2,2'-[(4-fluorobenzene-1,2-diyl)bis(oxy)]bis(5-nitrobenzonitrile) 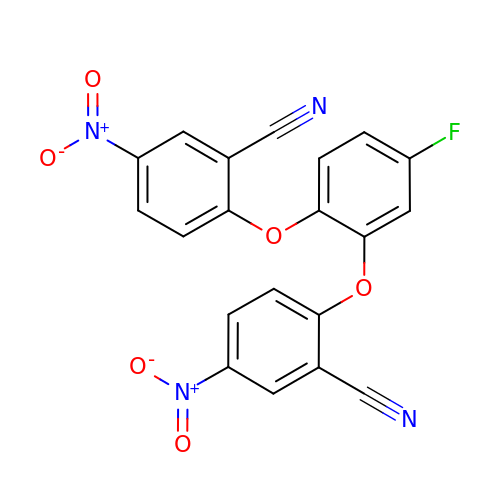| C20 H9 F N4 O6 | QHKCESVLSJWHFS-UHFFFAOYSA-N>VPPAIVVLIGPPGYVGKQYPITASDIVIGRSVESQVYIDDKSLSRSHAKFAVNGSEVSVIDLGSTNKTIVNGQVIPPLASCLLKNNDQIKTGNVIFKFLEKGSIEAMTNAAMYDRAQKDALTGAHSKGALL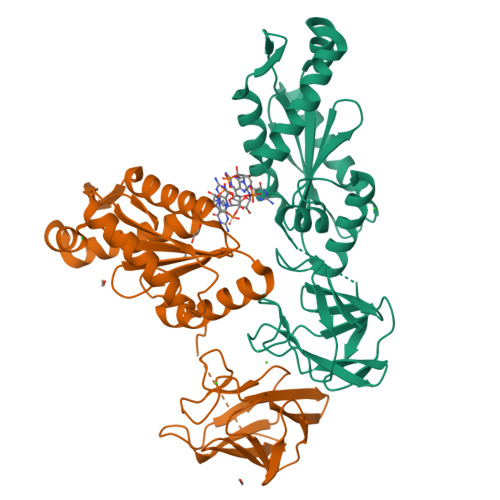DKGPEAMKRAEVLNEPFSLVTFDIDHFKKINDSYGHPGGDYVLKELCRIVITKLIRSNDFFARYGGEEFVLLLSGSPSKTAGEVGERIRQTIEAHDFTFEGKKIPVTISVGVATKLPNETEWTQVYDRADKALYQSKQGGRNRTTIVA[2x]N-[(3,5-dichlorophenyl)sulfonyl]-L-isoleucyl-N-hydroxy-L-norvalinamide | C17 H25 Cl2 N3 O5 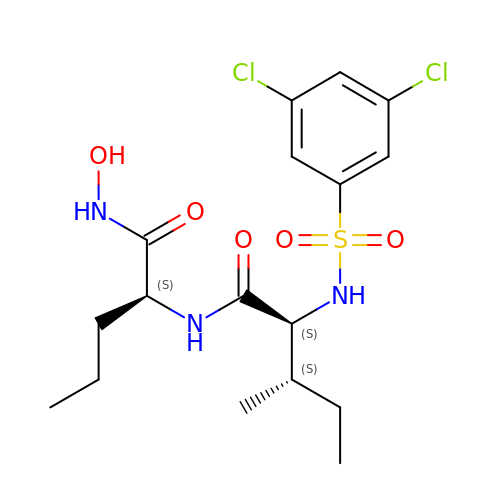S | VNYSFABAYGTWDO-LKTVYLICSA-N> MRLTQGCFSFLPDLTDAQIEKQVAYAMSRGWAMNVEWTDDPHPRNNYWELWGLPLFDIKDPATVMFELNEARKSCAAGYIRMNAFDASYGTESC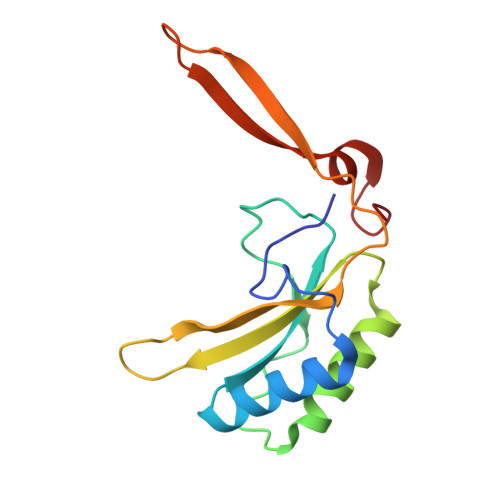VMSFLTNRPANEPGFYLDRTDGIGRQIIYSIKSYSVQANPEGSRY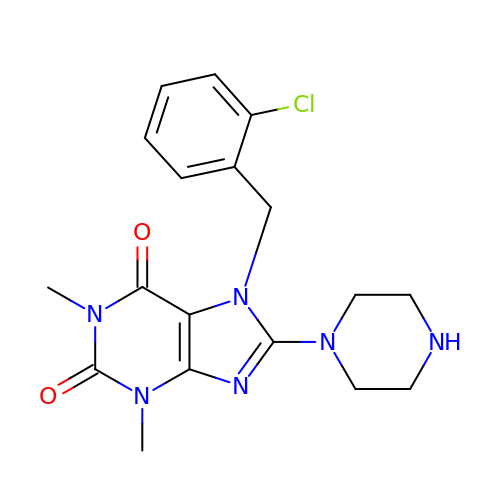7-(2-chlorobenzyl)-1,3-dimethyl-8-piperazin-1-yl-3,7-dihydro-1H-purine-2,6-dione | C18 H21 Cl N6 O2 | PDZWWGBRZISNRL-UHFFFAOYSA-N>MGSSHHHHHHSSGMADLSELLKEGTKEAHDRAENTQFVKDFLKGNIKKELFKLATTALYFTYSALEEEMERN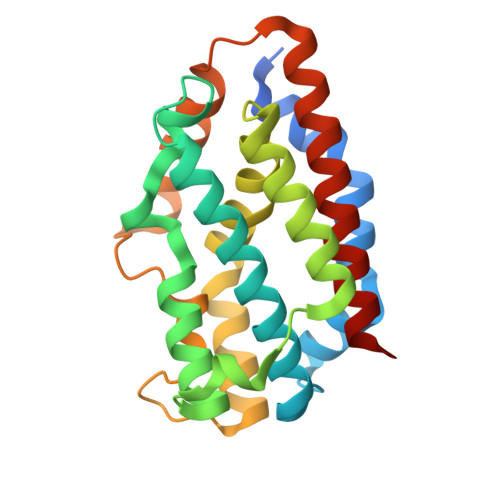KDHPAFAPLYFPMELHRKEALTKDMEYFFGENWEEQVQCPKAAQKYVERIHYIGQNEPELLVAHAYTRYMGDLSGGQVLKKVAQRALKLPSTGEGTQFYLFENVDNAQQFKQLYRARMNALDLNMKTKERIVEEANKAFEYNMQIFNELDQAGS[4x]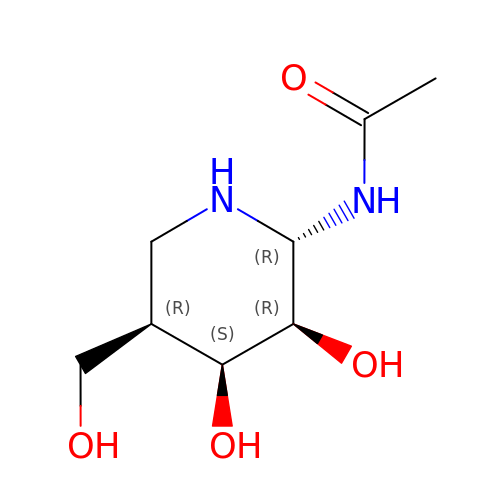(2R,3R,4S,5R)-2-ACETAMIDO-3,4-DIHYDROXY-5-HYDROXYMETHYL-PIPERIDINE | C8 H16 N2 O4 | IWVRQJNSUOIUFV-VGRMVHKJSA-N>[2x]MNRVDLSLFIPDSLTAETGDLKIKTYKVVLIARAASIFGVKRIVIYHDDADGEARFIRDILTYMDTPQYLRRKVFPIMRELKHVGILPPLRTPHHPTGKPVTGEYRQGLTVKRVKKGTLVDIGADKLALCREKLTVNRIMSFRVVRLGKEILIEPDEPEDRYWGYEVLDTRRNLAESLKTVGADVVVATSRNASPITSILDE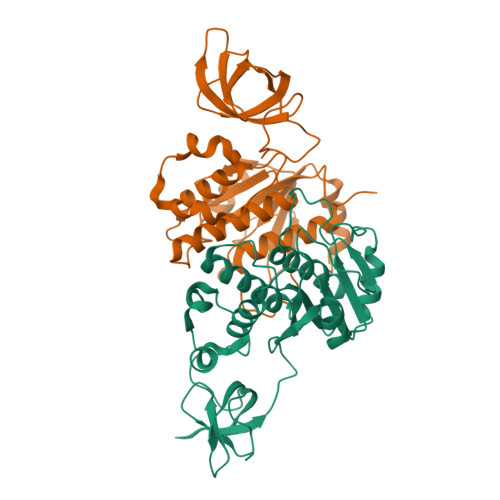VKTRMRGAREAAILFGGPYKGLPEIDADIWVNTLPGQCTETVRTEEAVLATLSVFNMLTQIDEKDE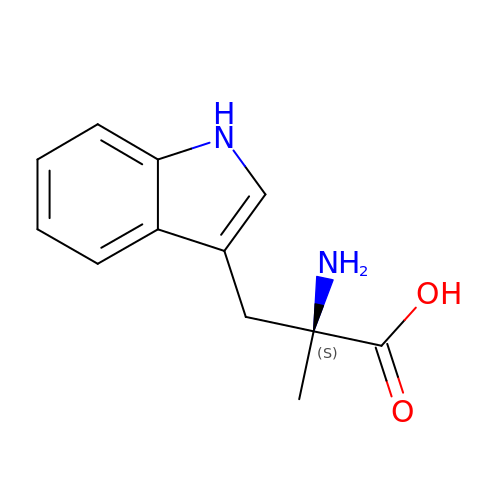alpha-methyl-L-tryptophan | C12 H14 N2 O2 | ZTTWHZHBPDYSQB-LBPRGKRZSA-N>MLPGTFFEVLKNEGVVAIATQGEDGPHLVNTWNSYLKVLDGNRIVVPVGGMHKTEANVARDERVLMTLGSRKVAGRNGPGTGFLIRGSAAFRTDGPEFEAIARFKWARAAL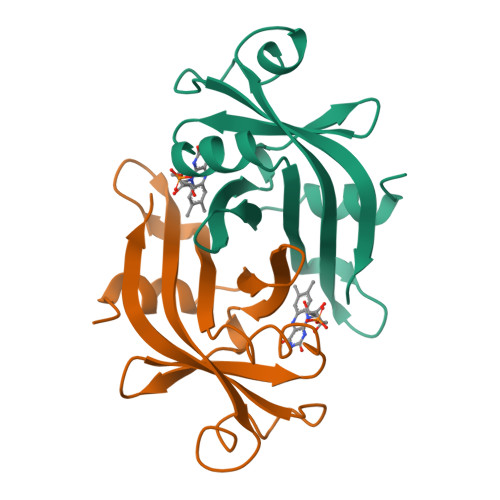VITVVSAEQTL[2x]> AKPFELLVSFLNTPKYGTFDPTPVVPVFFPFWFGMIVGDIGYALLFYLVGRWLSGYVKRNEPLVIDLFALKLKPQVIGKLVHILNWMVFWTVVWGVIYGEFFGTFLEHLGVFGTPEHPGLIPILIHRIDTAKTANLLILLSVAFGVVLVFFGLALRAYLGLKHRHMAHFWEGVGYLGGLVGVLALAASYLGNLQAGWLQGLMYLGFGVFLLAVLMSRIWLMIPEIFTQAGHILSHIRIYAVGAAGGILAGLLTDVGFALAERLGLLGVLLGLLVAGVLHLLILLLTTLGHMLQPIRLLWVEFFTKFGFYEENG;>SGGLDRGLIAVGMGLAVGLAALGTGVAQARIGAAGVGAIAEDRSNFGTALIFLLLPET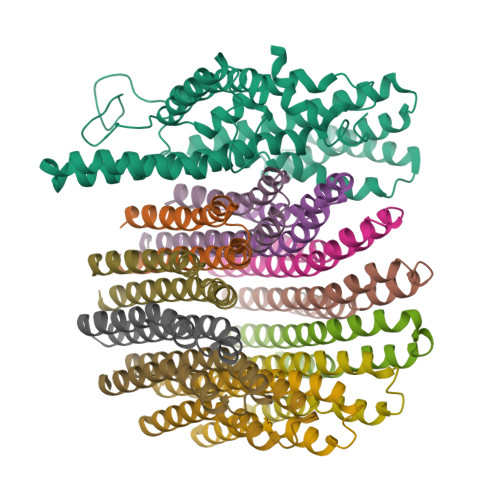LVIFGLLIAFILNGRL[12x]>SNAMSLDDIINNMIDKLKLLVHFDRISFLLLANETLKLSHVYPKGSHSLDIGSTIPKEQSLYWSALDQRQTIFRSLTDTQDNFYEKQYLAILDLKSILVIPIYSKNKRVGVLSIGRKQQIDWSLDDLA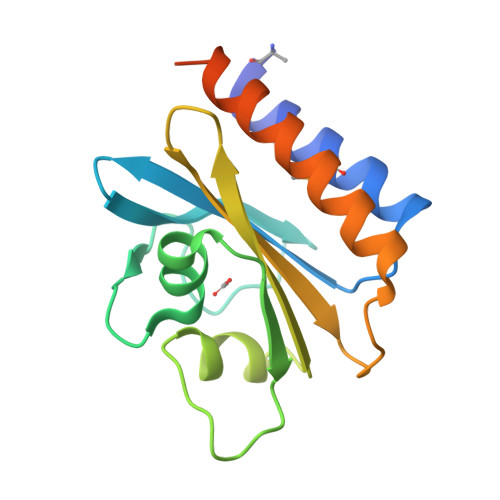FLEQLTDHLAVSIENVELYGQVLRSKQEWEDTFKAVD[2x]>[4x]SMLTELIASNRRSAAIHAFVDTGLSTHFKDGIYVDISELSRKSGVNYARFSRLCDFLVEMGVLVSNDNKFRLSDEC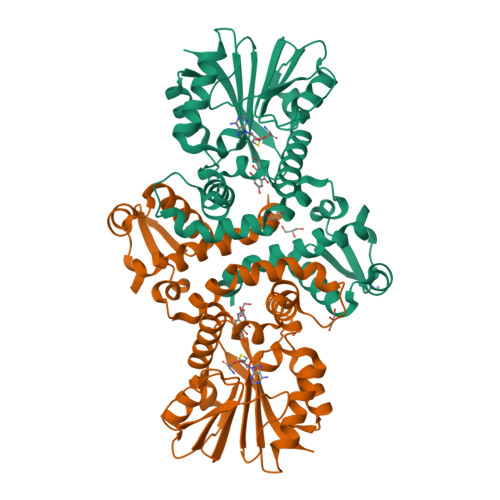HVFANPESFESFMIKLEICSHYSNAWLMYGKSLFEDDGKSAFEMAHGRPFFEYLDGNKFLKSNFDALMTRVSNLIVEKLLGIYDFNQHNRILDVGGGEGELLVRISEKVKGKHYAVLDRYSELPVSDNIDFINGNFLNSIPSGYDLYILKNVLNNWSDSDSILILENFRKAMDKNSSLLLINMVKEPEFSRSFDILMDVLFLGKERSFTEFEYLANQAGLVVQETKVIDQSYSPYSFIKLQIK> CEDVETHKPYGDGSGHAPGTVQVTSYEQIPGGVTLKFIAPTDEDLLYIKIKYTLDNGKEMEARASLYTDETTIEGFGNTNPKKLVISAVNKMEKEG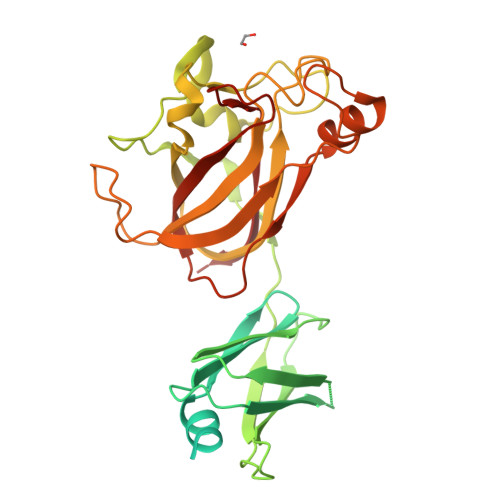EAIITEIVPGKPAYLTAIEEIEVNPTFGGIYIHTTNGGRNYLIFDVSTKDSKGNWNIEHTEYTSVKNIGFTLRGFSAEPHDFKVRVRDLYDNQSEEYLTTLTPLYEEKLDLTKFKTFYLANDIKMDNAGHTLESLFNGDHGLNSWNYAHGYDFNPSEFPVWFTFDMGQTAQLSRFTSWQRSMGGSYYYRAGAIKEWEVWGRSDLPSSDGSWDGWTKLADCESIKPSGWPTGSNSEEDITYASKGEEFEFLADIPPVRYIRFKILSTHDGAGLVVMQQLWFYGTPIQ1-(3,3-dimethylbutyl)-3-{2-fluoro-4-methyl-5-[7-methyl-2-(methylamino)pyrido[2,3-d]pyrimidin-6-yl]phenyl}urea | C23 H29 F N6 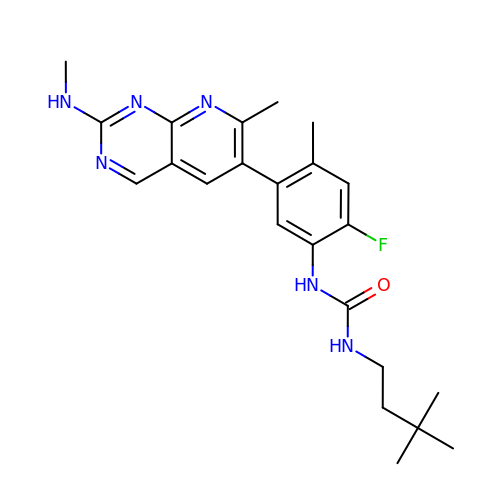O | HHCBMISMPSAZBF-UHFFFAOYSA-N> GHMTNLVAEPFAKLEQDFGGSIGVYAMDTGSGATVSYRAEERFPLCSSFKGFLAAAVLARSQQQAGLLDTPIRYGKNALVPWSPISEKYLTTGMTVAELSAAAVQYSDNAAANLLLKELGGPAGLTAFMRSIGDTTFRLDRWELELNSAIPGDARDTSSPRAVTESLQ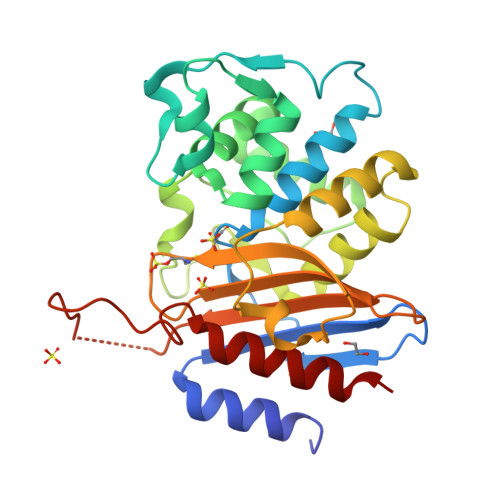KLTLGSALAAPQRQQFVDWLKGNTTGNHRIRAAVPADWAVGDKTGTCGVYGTANDYAVVWPTGRAPIVLAVYTRAPNKDDKHSEAVYTRAPNKDDKHSEAVIAAAARLALEGLG> PISPIETVPVKLKPGMDGPKVKQWPLTEEKIKALVEICTEMEKEGKISKIGPENPYNTPVFAIKKKDSTKWRKLVDFRELNKRTQDFWEVQLGIPHPAGLKKNKSVTVLDVGDAYFSVPLDEDFRKYTAFTIPSINNETPGIRYQYNVLPQGWKGSPAIFQSSMTKILEPFKKQNPDIVICQYMDDLYVGSDLEIGQHRTKIEELRQHLLRWGLTTPDKKHQKEPPFLWMGYE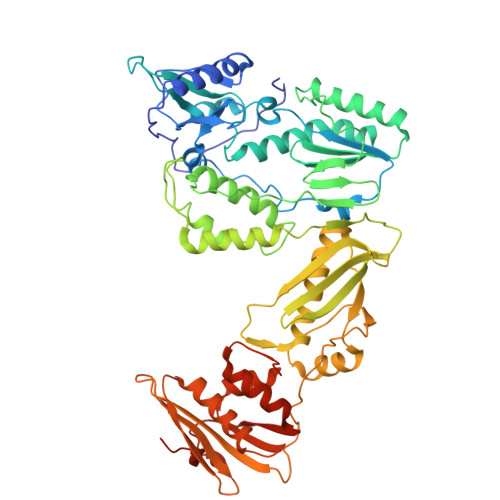LHPDKWTVQPIVLPEKDSWTVNDIQKLVGKLNWASQIYPGIKVRQLSKLLRGTKALTEVIPLTEEAELELAENREILKEPVHGVYYDPSKDLIAEIQKQGQGQWTYQIYQEPFKNLKTGKYARMRGAHTNDVKQLTEAVQKITTESIVIWGKTPKFKLPIQKETWETWWTEYWQATWIPEWEFVNTPPLVKLWYQLEKEPIVGAETFYVDGAANRETKLGKAGYVTNKGRQKVVPLTNTTNQKTELQAIYLALQDSGLEVNIVTDSQYALGIIQAQPDKSESELVNQIIEQLIKKEKVYLAWVPAHKGIGGNEQVDKLVSAGIRKIL> ALFEPY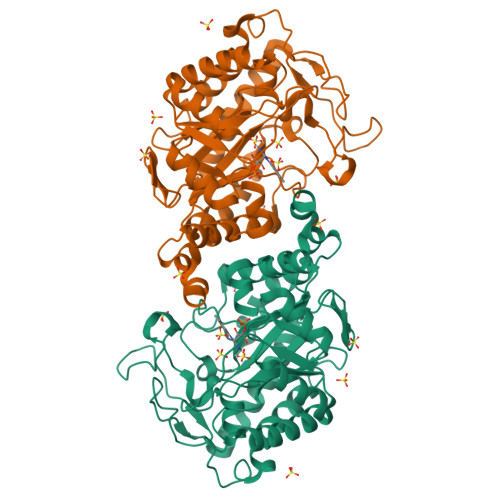TLKDVTLRNRIAIPPMCQYMAEDGMINDWHHVHLAGLARGGAGLLVVEATAVAPEGRITPGCAGIWSDAHAQAFVPVVQAIKAAGSVPGIQIAHAGRKASANRPWEGDDHIAADDTRGWETIAPSAIAFGAHLPKVPREMTLDDIARVKQDFVDAARRARDAGFEWIELHFAHGYLGQSFFSEHSNKRTDAYGGSFDNRSRFLLETLAAVREVWPENLPLTARFGVLEYDGRDEQTLEESIELARRFKAGGLDLLSVSVGFTIPDTNIPWGPAFMGPIAERVRREAKLPVTSAWGFGTPQLAEAALQANQLDLVSVGRAHLADPHWAYFAAKELGVEKASWTLPAPYAHWLE The neuraminidase inhibitors (NAIs) oseltamivir and zanamivir are the antiviral agents available in France to treat influenza A or B virus infections. The NA active site includes catalytic residues (R118, D151, R152, R224, E276, R292, R371, and Y406; N2 numbering) that interact directly with the sialic acid substrate and framework residues (E119, R156, W178, S179, D/N198, I222, E227, H274, E277, N294, and E425; N2 numbering) that stabilize the active site. NAs are divided into 3 phylogenic groups: influenza B viruses, group 1 (N1, N4, N5, and N8), and group 2 (N2, N3, N6, N7, and N9) from influenza A viruses. I221 (B NA numbering), I222 (N2 numbering), and I223 (N1 numbering) amino acids are highly conserved framework residues in NAs of influenza viruses.

We are the first to report influenza B viruses, isolated from an immunocompromised patient after prolonged oseltamivir treatment, with good fitness carrying a novel I221L substitution (B numbering) in NA that confers high-level resistance to oseltamivir. Sequencing of the NA gene in isolates revealed a unique mutation encoding an I221L substitution in NA at a level of 100% for isolates from a NPA obtained on D34 and a nasal swab specimen obtained on D40 and at a level of 80% for the isolate from a BAL obtained on D42. Analysis of HA and NA genes revealed that the only difference between oseltamivir-resistant and oseltamivir-susceptible isolates was the mutation conferring the I221L substitution in the NA gene. We used X-ray crystallography to understand the structural basis of resistance to oseltamivir conferred by NA carrying the I221L substitution. The Km revealed that the I221L NA variant had a 1.9 times lower affinity for the MUNANA substrate, and the Ki values for oseltamivir carboxylate and zanamivir showed affinities that were around 84 and 51 times lower, respectively, than that for wild-type NA. Moreover, the NA I221L substitution does not impair virus replicative fitness.

>[2x]MLPSTIQTLTLFLTSGGVLLSLYVSALLSYLLYSDILLKFSPTEITAPTMSLDCANASNVQAVNRSATKGVTFLLPEPEWTYPRLSCPGSTFQKALLISPHRFGETKGNSAPLIIREPFIACGPNECKHFALTHYAAQPGGYYNGTRGDRNKLRHLISVKLGKIPTVENSIFHMAAWSGSACHDGKEWTYIGVDGPDNDALLKVKYGEAYTDTYHSYANKLLRTQESACNCIGGNCYLMITDGSASGVSECRFLKIREGRIIKEIFPTGRVKHTEECTCGFASNKTIECACRDNSYTAKRPFVKLNVETDTAEIRLMCTDTYLDTPRPDDGSITGPCESNGDKGSGGIKGGFVHQRMESKIGRWYSRTMSKTERMGMGLYVKYDGDPWADSDALAFSGVMVSMKEPGWYSFGFEIKDKECDVPCIGIEMVHDGGKETWHSAATAIYCLMGSGQLLWDTVTGVDMAL> MAKREPIHDNSIRTEWEAKIAKLTSVDQATKFIQDFRLAYTSPFRKSYDIDVDYQYIERKIEEKLSVLKTEK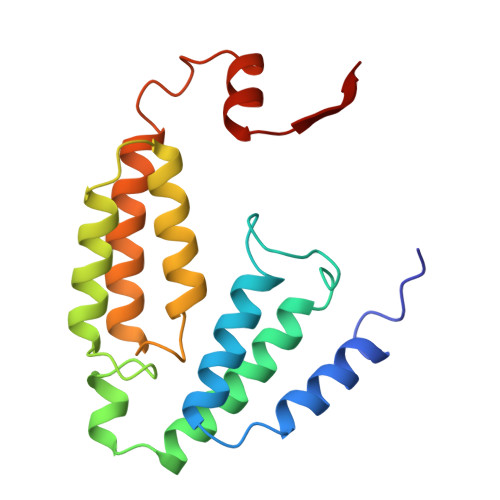LPVADLITKATTGEDAAAVEATWIAKIKAAKSKYEAEAIHIEFRQLYKPPVLPVNVFLRTDAALGTVLMEIRNTDYYGTPLEGLRKERGVKVLHLQA>[2x]GSMQQIPQCAGCNQHILDKFILKVLDRHWHSSCLKCADCQMQLADRCFSRAGSVYCKEDFFKRFGTKCTACQQGIPPTQVVRKAQDFVYHLHCFACIICNR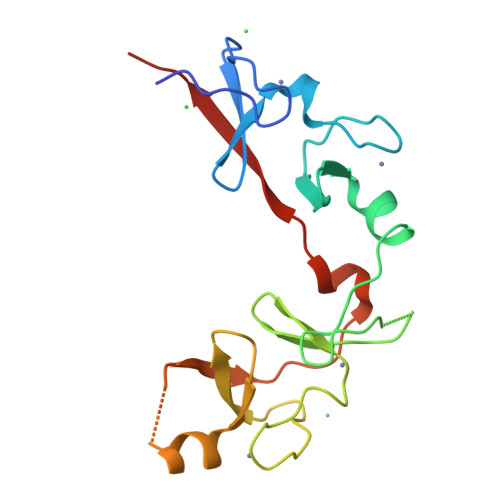QLATGDEFYLMEDGRLVCKEDYETAKQGGSGGHMGSGGGTPLVAGSPIGHENAVQGSAVEVQTYQPPW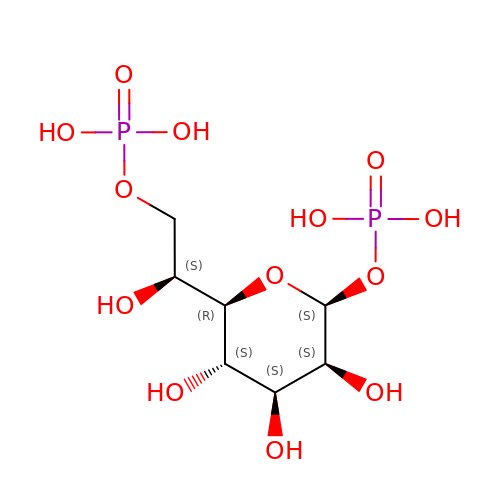1,7-di-O-phosphono-L-glycero-beta-D-manno-heptopyranose | C7 H16 O13 P2 | LMTGTTLGDUACSJ-QQABCQGCSA-N> ENIEVHMLNKGAEGAMVFEPAYIKAN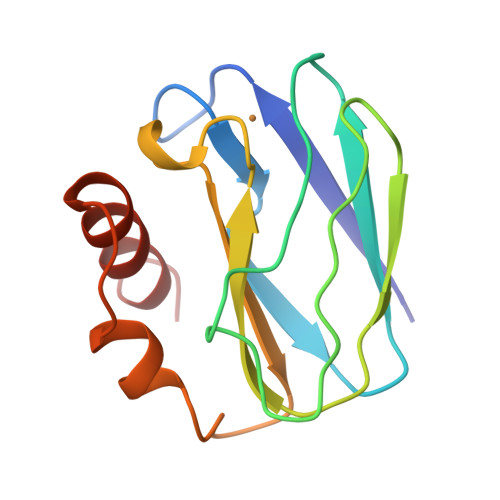PGDTVTFIPVDKGHNVESIKDMIPEGAEKFKSKINENYVLTVTQPGAYLVKCTIHYAMGMIALIAVGDSPANLDQIVSAKKPKIVQERLEKVIASAK>[2x]TAHRFLFVSTPVGPLGSGRGGGVELTLPNLAKALTQR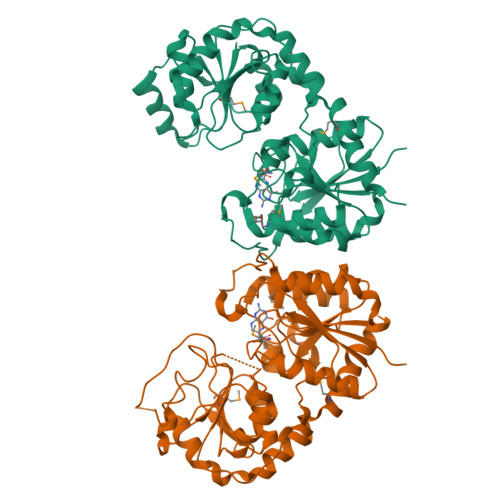GHQVSVLAPAGSVLPDLPLETVPGTWQSTAQSHGRATPAEIPAESVLARLWDRAHQQQADFDLILNFAYDWLPLYLTPFFKTPVAHLISMGSLSEVMDQAIATSLDRYPGSIAVHSLAQAATFPFGDRCLCIGNALDLAAYGFNPEPEPVLGWVGRIAPEKGLEDAIQAAQQAGLPLRVWGALTEPDYWQRLQQQFGDRAVSYQGFVSTDELQRGLGRCQGLLMTPKWVEAFGNVAIEALACGLPVIAYARGGPLEIIEQGKSGWLVEPDQQAALVNAIGQLSSLDRAYCRAQAEARFSLAAMGQRLEAWLLPLLSR> PISPIETVPVKLKPGMDGPKVKQWPLTEEKIKALVEICTEMEKEGKISKIGPENPYNTPVFAIKKKDSTKWRKLVDFRELNKRTQDFWEVQLGIPHPAGLKKKKSVTVLDVGDAYFSVPLDEDFRKYTAFTIPSINNETPGIRYQYNVLPQGWKGSPAIFQSSMTKILEPFRKQNPDIVIYQYMDDLYVGSDLEIGQHRTKIEELRQHLLRWGLTTPDKKHQKEPPFLWMGYELHPDKWTVQPIVLPEKDSWTVNDIQKLVGKLNWASQIYPGIKVRQLCKLLRGTKALTEVIPLTEEAEL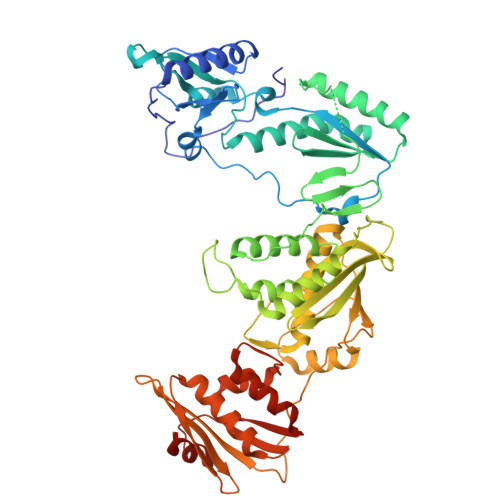ELAENREILKEPVHGVYYDPSKDLIAEIQKQGQGQWTYQIYQEPFKNLKTGKYARMRGAHTNDVKQLTEAVQKITTESIVIWGKTPKFKLPIQKETWETWWTEYWQATWIPEWEFVNTPPLVKLWYQLEKEPIVGAETFYVDGAANRETKLGKAGYVTNRGRQKVVTLTDTTNQKTELQAIYLALQDSGLEVNIVTDSQYALGIIQAQPDQSESELVNQIIEQLIKKEKVYLAWVPAHKGIGGNEQVDKLVSAGIRKVL> ILGGREAEAHARPYMASVQLNGAHLCGGVLVAEQWVLSAAHCLEDA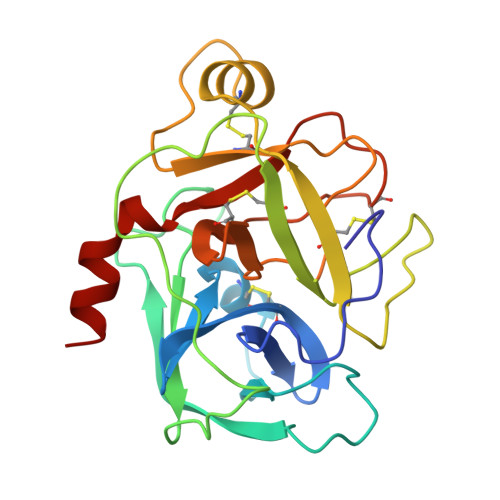ADGKVQVLLGAHSLSQPEPSKRLYDVLRAVPHPDYQPDTIDHDLLLLQLSEKATLGPAVRPLPWQRVDRDVAPGTLCDVAGWGIVNHAGRRPDSLQHVLLPVLDRATCNRRTHHDGAITERLMCAESNRRDSCKGDSGGPLVCGGVLEGVVSWGSRVCGNRKKPGIYTRVASYAAWIDSVLA> MGSDKIHHHHHHENLYFQGKVEYIEDPS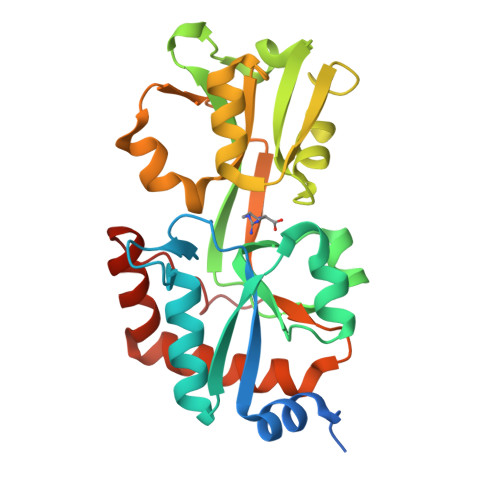WSKVQVKSALVIGVSDFVPILSFRNEKNEIVGYDIDIFTELCRRLGIHPIFYPIQWAQKEILLNTGVIDCIASGFSVTEERKQHYRMCTPYLQNAKIVVTLAGRGYQTLAQLQNRTIAVEADTAGDEALLNVEALKDHVIIKAMATIDQLYEALDSGTCDAIVVDLIYSLDTLDKNPQYSIINEAISTEYYTFAFRQADASLVAKIESVLAEMNEDETIPNFSRKWFGSNLSILNVRF>[2x]MPPRKELVGNKWFIENYENETESLVIDANKDESIFIGKCSQVLVQIKGKVNAISLSETESCSVVLDSSISGMDVIK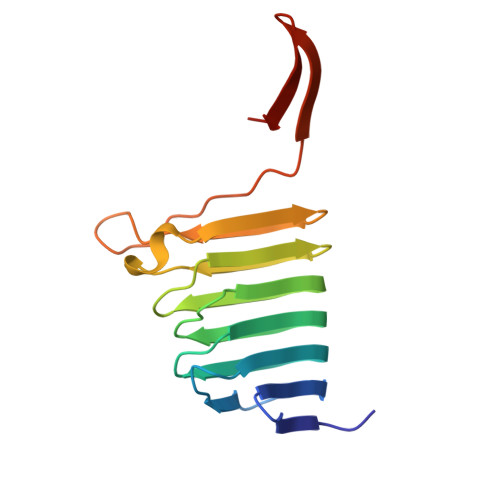SNKFGIQVNHSLPQISIDKSDGGNIYLSKESLNTEIYTSCSTAINVNLPIGEDDDYVEFPISEQMKHSFADGKFKSAVFEHAG>[2x]PDVDECALGANPCEHAGKCLNTLGSFECQCLQGYTGPRCEIDVNECISNPCQ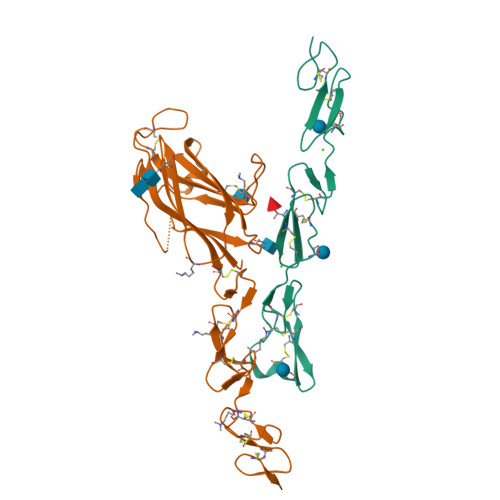NDATCLDQIGEFQCICMPGYEGVYCEINTDECASSPCLHNGRCVDKINEFLCQCPKGFSGHLCQSG;>[2x]GSSSIFQLRLQEFANERGMLANGRPCEPGCRTFFRICLKHYQATFSEGPCTFGNVSTPVLGTNSFVIRDKNSGSGRNPLQLPLNFTWPGTFSLNIQAWHTPGDDLRPETSPGNSLISQIIIQGSLAVGKNWKSDEQNNTLTRLRYSYRVVCSDNYYGDSCSRLCKKRDDHFGHYECQPDGSPSCLPGWTGKYCDQPICLSGCHEQNGYCSKPDECNCRPGWQGPLCNEAA> NDQPFAWQVASLSERYQEQFDIGAAVEPYQLEGRQAQILKHHYNSLVAENAMKPVSLQPREGEWNWEGADKIVEFARKHNMELRFHTLVWHSQVPEWFFIDENGNRMVDETDPEKRKANKQLLLERMENHIKTVVERYKDDVTSWDVVNEVIDDDGGLRESEWYQITGTDYIKVAFETARKYGGEEAKLYINDYNTENPSKRDDLYNLVK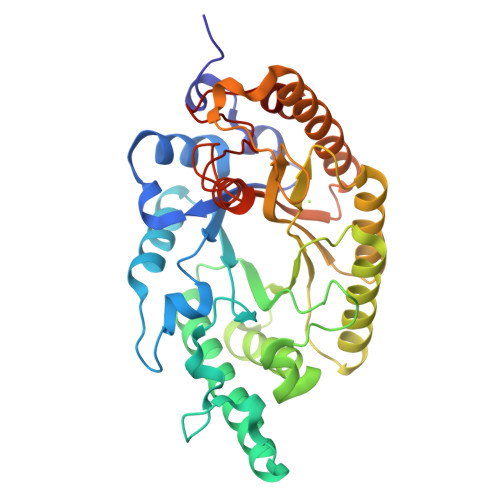DLLEQGVPIDGVGHQSHISIGRPSIEDTRASFEKFTSLGLDNQVTELDMSLYGWPPTGAYTSYDDIPEELFQAQADRYDQLFELYEELSATISSVTFWGIADNHTWLDDRAREYNNGVGVDAPFVFDHNYRVKPAYWRIID>GPLGSMAGTFKIHAYTEGGKPLRTIYLPKLLKKVFLDVVKPNTKKNLETCGILCGKLRQNAFFITHLVIPLQEATSDTCGTTDEASLFEFQDKHNLLTLGWIHTHPTQTCFMSSVDLHTHCSYQLMLPE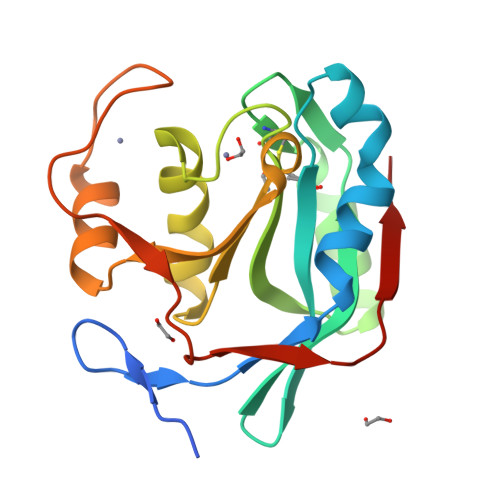AIAIVMAPSKNTSGIFRLLDPEGLQTIVKCRKPGLAHPHEGKVYTMVAQPGHVREINSKLQVVDLRVK[2x]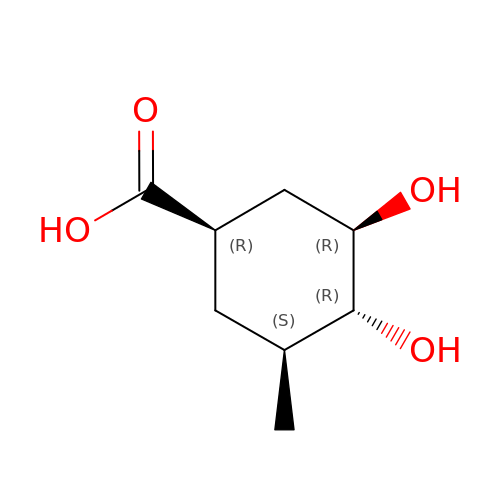(1~{R},3~{S},4~{R},5~{R})-3-methyl-4,5-bis(hydroxyl)cyclohexane-1-carboxylic acid | C8 H14 O4 | OBDLOCPYNMEWCH-BDVNFPICSA-N>[2x]MAP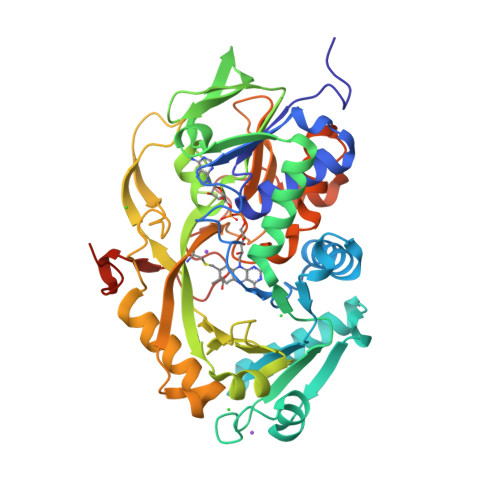SRANTSVIVVGGGGTIGSSTALHLVRSGYTPSNVTVLDAYPIPSSQSAGNDLAKIMGVSLRNPVDLQLALEARQMWNEDELFKKFFHNTGRLDCAHGEKDIADLKSGYQALVDAGLDATNEWLDSEDEILKRMPLLSRDQIKGWKAIFSKDGGWLAAAKAINAVGEYLRDQGVRFGFYGAGSFKAPLLAEGVCIGVETVDGTRYYADKVVLAAGAWSPTLVELHEQCVSKAWVYGHIQLTPEEAARYKNSPVVYNGDVGFFFEPNEHGVIKVCDEFPGFTRFKMHQPFGAKAPKRISVPRSHAKHPTDTIPDASDVSIRRAIATFMPQFKNKKMFNQAMCWCTDTADAALLICEHPEWKNFVLATGDSGHSFKLLPNIGKHVVELLEGTLADDLAHAWRWRPGSGDALKSRRSAPAKDLADMPGWNHDKPRANLLEHHHHHH> MNNNKAEADTSSSMADPETRPTYTTHHLAIPSGVTQDEFDELKQSVVEFHTYQLSQNQCSSLLAQRIRAPNDVVWSIVRRFDQPQTYKHFIKSCSVSDNFTMAVGSTRDVNVISGLPAATSTERLDILDDDRQVTGFSIIGGEHRLRNYRSVTSVHGFNRDGAICTVVLESYVVDVPEGNTEEDTRLFADTVVKLNLQKLVSVAESQVI;> RSVYELDCIPLWGTVSIQGNRSEMEDAFAVSPHFLKLPIKMLMGDHEGMSPSLTHLTGHFFGVYDGHGGHKVADYCRDRLHFALAEEIERIKDELCKRNTGEGRQVQWDKVFTSCFLTVDGEIEGKIGRAVVGSSDKVLEAVASETVGSTAVVALVCSSHIVVSNCGDSRAVLFRGKEAMPLS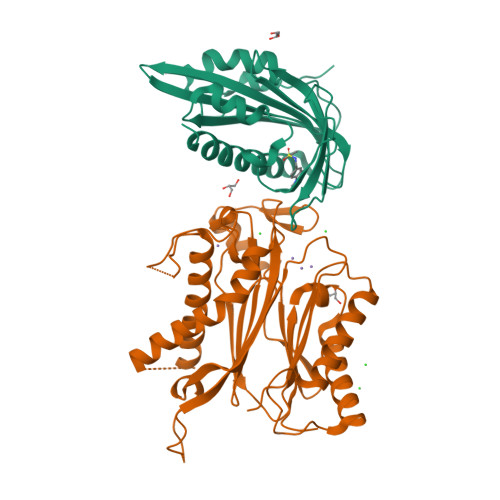VDHKPDREDEYARIENAGGKVIQWQGARVFGVLAMSRSIGDRYLKPYVIPEPEVTFMPRSREDECLILASDGLWDVMNNQEVCEIARRRILMWHKKNGAPPLAERGKGIDPACQAAADYLSMLALQKGSKDNISIIVIDLKAQRKFKTRT(4R)-4-(2-carboxyethyl)imidazolidin-2-iminium | C6 H12 N3 O2 | 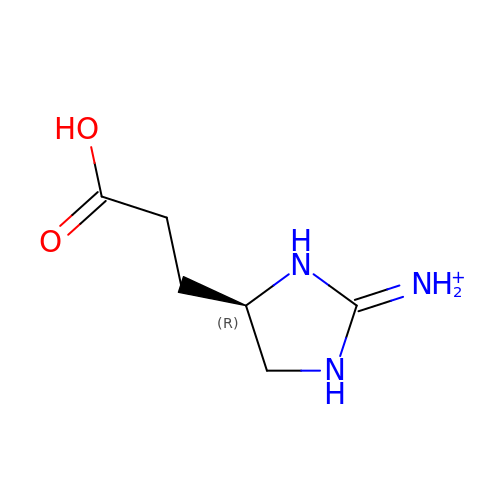XWJJYUBXTJRSEQ-SCSAIBSYSA-O> MSDNEGSVPTEGIDYGDTMVVWPSTGRIPGGDVKPGGSSGLAPSMPPGWGDYSPQGIALVQSVLFPGIIRRIILDKELEEGDWSGWSVSVHSPWGNEKVSAARTVLENGLRGGLPEPSRPAAVSFARLEPASGNEQKIIRLMVTQQLEQVTDIPASQLPAAGNNVPVKYRLTDLMQNGTQYMAIIGGIPMTVPVVDAVPVPDRSRPGTNIKDVYSAPVSPNLPDLVLSVGQMNTPVRSNPEIQEDGVISETGNYVEAGYTMSSNNHDVIVRFPEGSGVSPLYISAVEILDSNSLSQRQEAENNAKDDFRVKKEQENDEKTVLTKTSEVIISVGDKVGEYLGDKYKALSREIAENINNFQGKTIRSY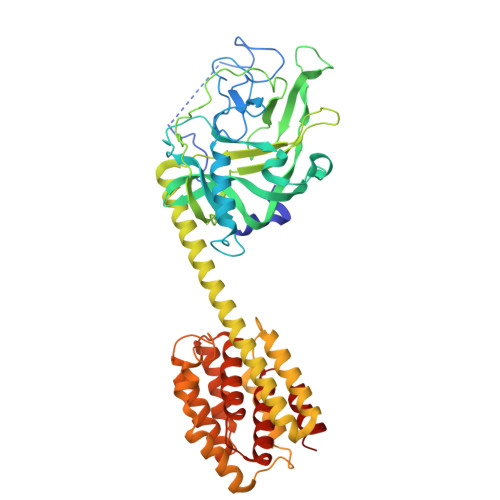DDAMSSINKLMANPSLKINATDKEAIVNAWKAFNAEDMGNKFAALGKTFKAADYAIKANNIREKSIEGYQTGNWGPLMLEVESWVISGMASAVALSLFSLTLGSALIAFGLSATVVGFVGVVIAGAIGAFIDDKFVDELNHKIIK>[2x]AASSPLLIGDSVMVDIGNVFTKKIPNAQIDGKVGRQLVDATPIVKSQYKDYAAAGQKVVVE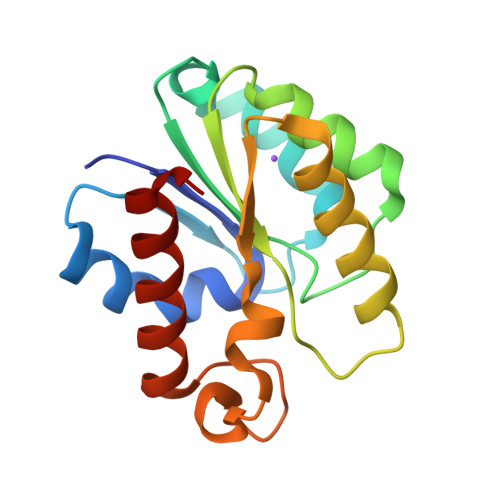LGTNGAFTKDQLNELLDSFGKADIYLVSIRVPRDYEGRINKLIYEAAEKRSNVHLVDWYKASAGHPEYFAYDGIHLEYAGSKALTDLIVKTMETHATN(8S)-N-cyclopropyl-5-[(2-methoxypyridin-3-yl)amino]-7-(methylamino)pyrazolo[1,5-a]pyrimidine-3-carboxamide | 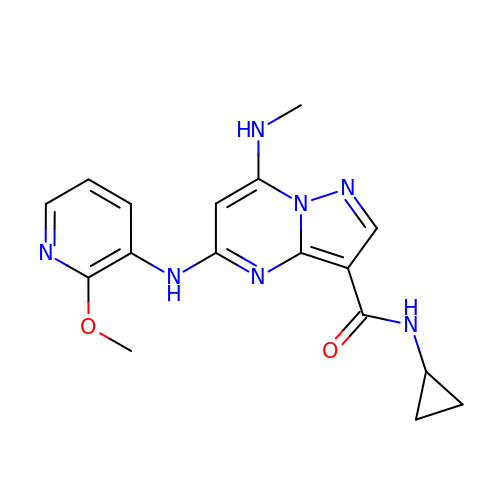C17 H19 N7 O2 | HANGACPWNQHVPZ-UHFFFAOYSA-N7-(diethylamino)chromen-2-one | C13 H15 N O2 | 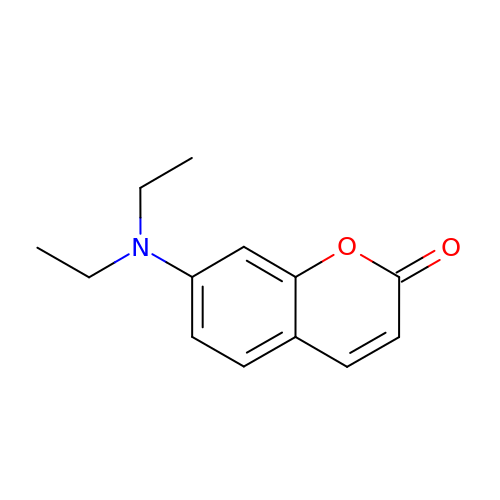QXAMGWKESXGGNV-UHFFFAOYSA-N> MASHLASIYGTEQDKVNCSFYYKIGACRHGERCYRKHVKPNFSQTILCPNMYKNPIHEPNGKKFTQRELAEQFDAFYEDMFCEFSKYGEVEQLVVCDNVGDHLVGNVYVRFKYEESAQNAIDDLNSRWYSQRPVYAELSPVTDFREACCRQHETSECQRGGLCNFMHAKKPSPQLLRDLVLAQRKYLAL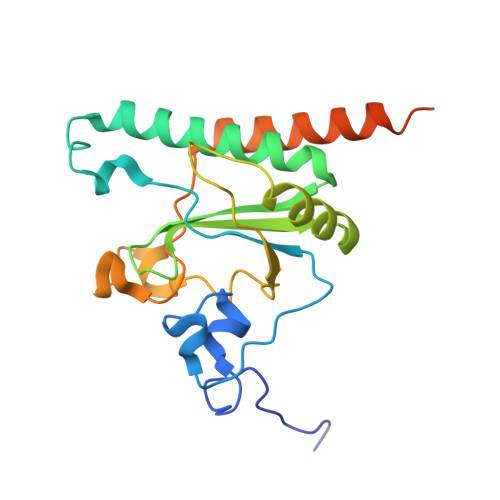NAAEEMKKEPNSDSTNRWVSVTAERKN> AACC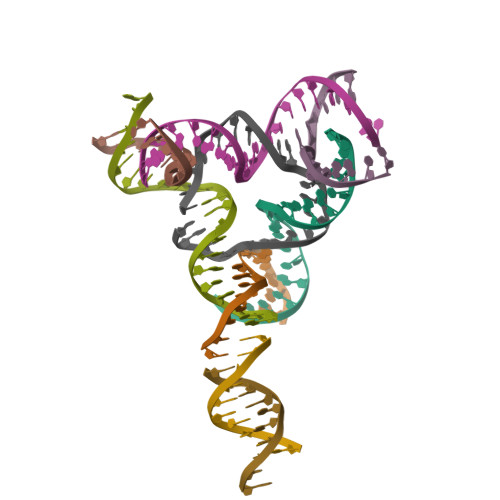TACTTGGCAGGACGACT;> TCTGATGTGGTAGG;> TTAGTCGTGGCTCG;> CACGAGCCTGATCGGACAAGA;> TGTCTTGTGGTCGC;> ACGCGACCTGTACGGACATCA;> ACACCGATCACCTGCCACCGT;> GTTAGCAGAG;> GACTCTGCTA>[6x]EHQAIAKMRTMIEGFDDISHGGLPIGRSTLVSGTSGTGKTLFSIQFLYNGIIEFDEPGVFVTFEETPQDIIKNARSFGWDLAKLVDEGKLF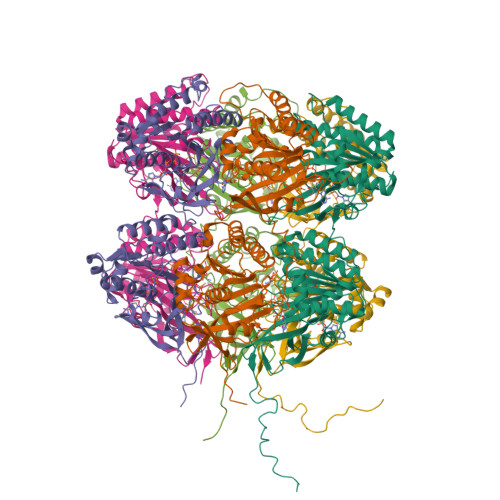ILDASPDPEGQEVVGGFDLSALIERINYAIQKYRARRVSIDSVTSVFQQYDASSVVRRELFRLVARLKQIGATTVMTTERIEEYGPIARYGVEEFVSDNVVILRNVLEGERRRRTLEILKLRGTSHMKGEYPFTITDHGINIFPLGAMRLTQRSSNVRVSSGVVRLDEMCGGGFFKDSIILATGATGTGKTLLVSRFVENACANKERAILFAYEESRAQLLRNAYSWGMDFEEMERQNLLKIVCAYPESAGLEDHLQIIKSEINDFKPARIAIDSLSALARGVSNNAFRQFVIGVTGYAKQEEITGLFTNTSDQFMGVHSITDSHISTITDTIILLQYVEIRGEMSRAINVFKMRGSWHDKAIREFMISDKGPDIKDSFRNFERIISGSPTRITVDEKSELSRIVRGVQEKGPESHHHHHH> MALSEIETRHSEIIKLENSIRELHDMFMDMAMLVESQGEMIDRIEYNVEHA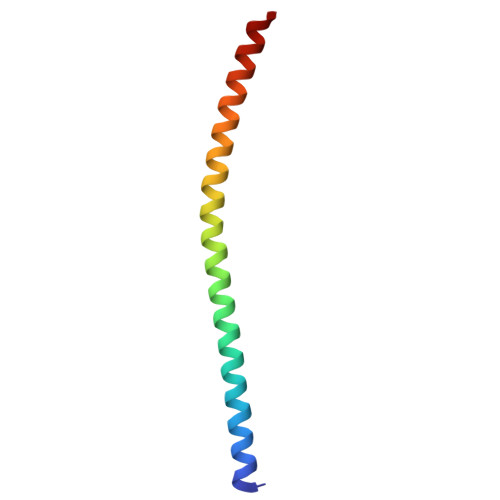VDYVERAVSDTKKAVK>[5x]MTQELGNANFENFIGATEGFSEIAYQFTSHILTLGYAV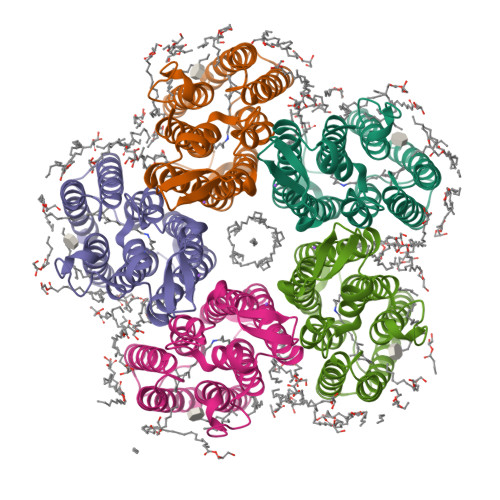MLAGLLYFILTIKNVDKKFQMSNILSAVVMVSAFLLLYAQAQNWTSSFTFNEEVGRYFLDPSGDLFNNGYRYLNWLIDVPMLLFQILFVVSLTTSKFSSVRNQFWFSGAMMIITGYIGQFYEVSNLTAFLVWGAISSAFFFHILWVMKKVINEGKEGISPAGQKILSNIWILFLISWTLYPGAYLMPYLTGVDGFLYSEDGVMARQLVYTIADVSSKVIYGVLLFNLAITLSKNKELVEANSLEHHHHHH>GSLANEKLSQLQKQLEEANDLLRTESDTAVRLRKSHTEMSKSISQLESLNRELQERNRILENSKSQTDKDYYQLQAILEAERRDRGHDSEMIGDLQARITSLQEEVKHLKHNLEKVEGERKEAQDMLNHSEKEKNNLEIDLNYKLKSLQQRLEQEVNEHKVT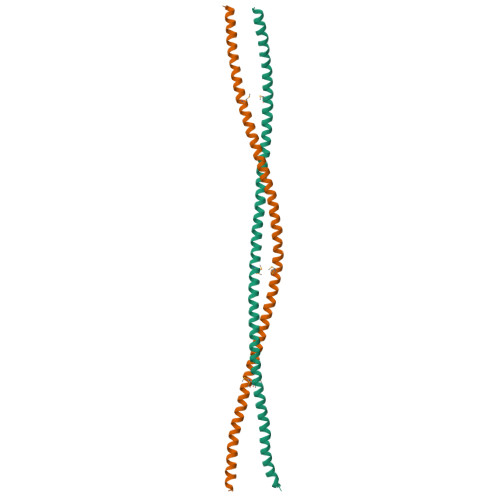KARLTD[4x]> MSGHHHHHHVILEANKIRKSYGNKLNKQEVLKGIDIHIEKGEFVSIMGASGSGKTTLLNVLSSIDQVSHGTIHINGNDMTAMKEKQLAEFRKQHLGFIFQDYNLLDTLTVKENILLPLSITKLSKKEANRKFEEVAKELGIYELRDKYPNEISGGQKQRTSAGRAFIHDPSIIFADQ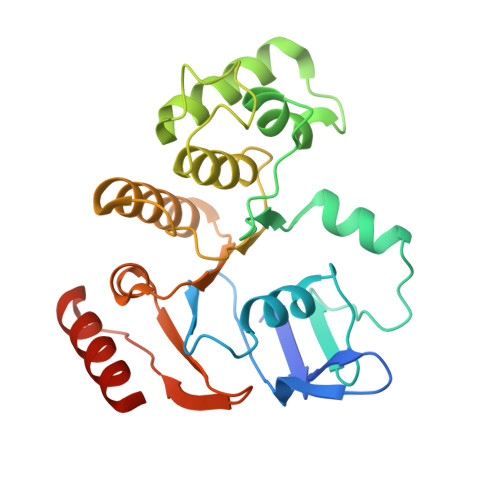PTGALDSKSASDLLNKLSQLNQKRNATIIMVTHDPVAASYCGRVIFIKDGQMYTQLNKGGQDRQTFFQDIMKTQGVLGGVQHEH> MEKKWWKEAVAYQIYPRSFMDSNGDGIGDIQGVISKLDYLSDLGIDVIWICPIYQSPNDDNGYDISDYKDIMKDFGTMEDFDELLDEVHHRGMKLIMDLVINHTSDEHPWFLESRSAKENPYRDYYIWHEGKDGKEPNNWESIFSGSAWEFDEKTKEYYMHVFSKKQPDLNWENEKVRHELYEMVNWWLDKGIDGFRVDAISHIKKVAGFPDLPNPEKLDYVPSFEGHMNRPGIQEHLKELKEKTFAKYDIMTVGEANGVTSDSADEWVAEDGGNFNMIFQFEHMGLWDKGEEKPLDLIELKTILTNWQNGLEKINGWNALYLENHDQIRSVNKFGSTAYRVESAKCLAALYFLMKGTPFIYQGQELGMTNVKFDSIDDYDDVGMINYYRIQREKGDSHDEIMKVIWETGRDNSRTPMQWNTEKNAGFSTGNPWMKVNPN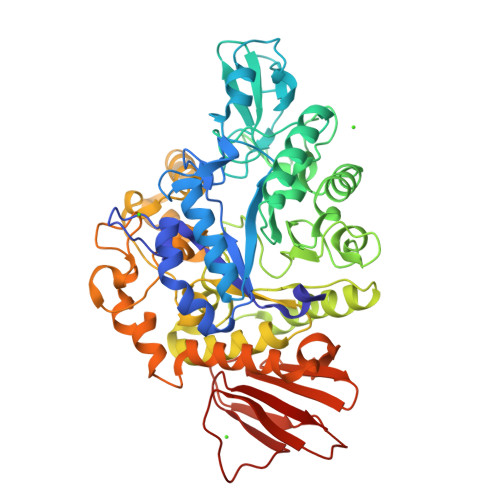YVDINVEEQKSDKNSVLNFYKQLIKIRKQHDVLVYGTYKLLAEEDSAIYAYTRTLEGKTAVVICNMSPNNQTFEFPSESSFTNIEVLIHNYPLDKNETLEQCTLHPYETRVYLIS>GSKPFSLPILTLSELTNSRFPVPIDSLFTAQNNVLQVQCQNGRCTLDGELQGTTQLLPTGICAFRGRVTAQINQRDRWHMQLQNLNGTTYDPTDDVPAPLGTPDFKGVVFGM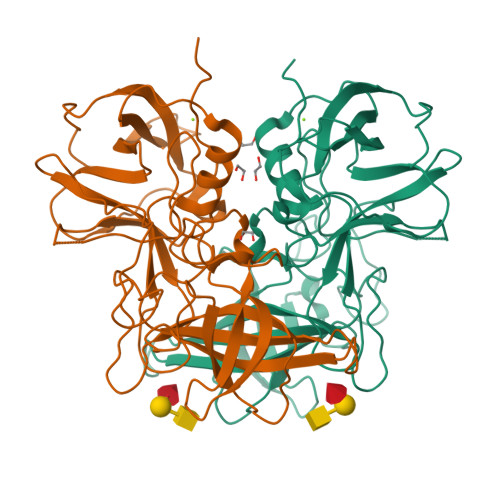VSQRNVGNDAPGSTRAQQAWVSTYSPQFVPKLGSVNLRISDNDDFQFQPTKFTPVGVNDDDDGHPFRQWELPNYSGELTLNMNLAPPVAPNFPGEQLLFFRSFVPCSGGYNQGIIDCLIPQEWIQHFYQESAPSQSDVALIRYVNPDTGRTLFEAKLHRSGYITVAHSGDYPLVVPANGHFRFDSWVNQFYSLAPM[2x]> XXXXXXXXXXXXXXXXXXXXXXXXXXXXXSYPVSLNINLNSDKLVFPAVTICTLNPYRYPEIKEELEELDRITEQTLFDLYKYSSFTTLVAGSRSRADLRGTLPHPLQALAVPPPPHGAAAAASVASSLRDNNPQVDWKDWKIGFQLCNQNKSDCFYQTYSSGVDAVAEWYAFHYINILSRLPETLPSLEEDTLGNFIFACRFNQVSCNQANYSHFHHPMYGNCYTFNDKNNSNLWMSSMPGINNGLSLMLRAEQNDFIPLLSTVTGARVMVHGQDEPAFMDDGGFNLRPGVETSISMRKETLDRLGGDYGDCTKNGSDVPVENLYPSKYTQQVCIHSCFQESMIKECGCAYIFYPRPQNVEYCDYRKHSSWGYCYYKLQVDFSSDHLGCFTKCRKPCSVTSYQLSAGYSRWPSVTSQEWVFQMLSRQNNYTVNNKRNGVAKVNIFFKELNYKTNSESPSVTXXX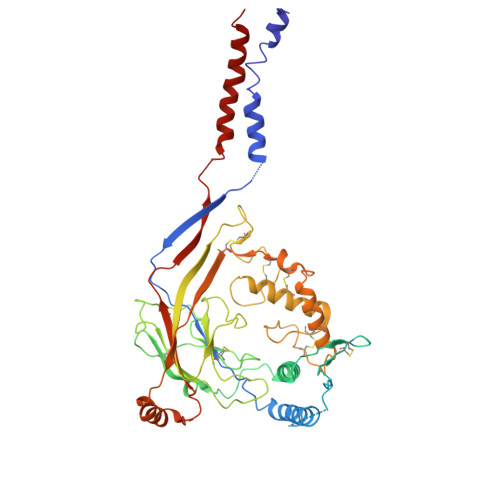XXXXXXXXXXXXXXXXXXXXXXXX> MLYEEDYKLALEAFKKVFNALTHYGAKQAFRSRARDLVEEIYNSGFIPTFFYIISKAELNSDSLDSLISLFSSDNAILRGSDENVSYSAYLFIILYYLIKRGIIEQKFLIQALRCEKTRLDLIDKLYNLAPIISAKIRTYLLAIK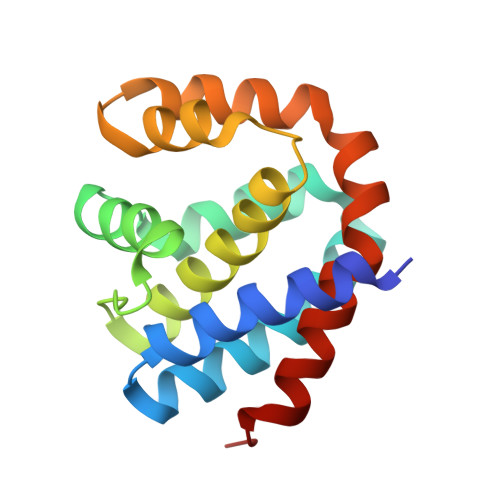RLSEALIEAR> CPQGKYIHPQNNSICCTKCHKGTYL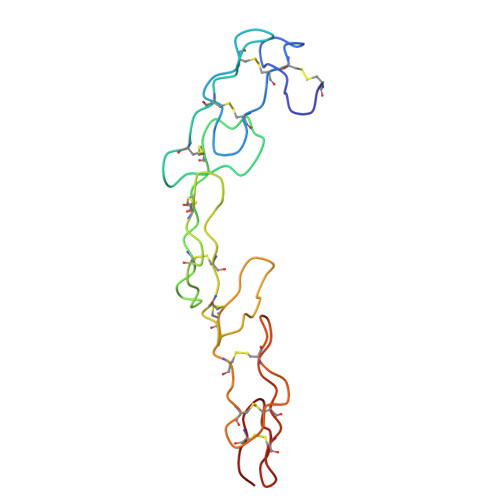YNDCPGPGQDTDCRECESGSFTASENHLRHCLSCSKCRKEMGQVEISSCTVDRDTVCGCRKNQYRHYWSENLFQCFNCSLCLNGTVHLSCQEKQNTVCTCHAGFFLRENECVSC Spermidine is a polyamine molecule that performs various cellular functions, such as DNA and RNA stabilization, autophagy modulation, and eIF5A formation, and is generated from putrescine by aminopropyltransferase spermidine synthase (SpdS). During synthesis, the aminopropyl moiety is donated from decarboxylated S-adenosylmethionine to form putrescine, with 5′-deoxy-5′-methylthioadenosine being produced as a byproduct. Spermidine synthase (SpdS; EC 2.5.1.16) is a major type of aminopropyltransferase that converts putrescine into spermidine. In addition, SpdS contains a structural feature known as the gate-keeping loop, which is located in the vicinity of the entrance to the active site.

Here, we determined the crystal structure of an apo-form of SpdS from Kluyveromyces lactis (KlSpdS) at 1.9 Å resolution. KlSpdS exists as a dimer in the asymmetric unit, and each monomer in the dimeric KlSpdS is positioned with two-fold symmetry. Each KlSpdS monomer consists of three domains: an N-terminal domain (residues 4–66), a central catalytic core domain (residues 67–250), and a C-terminal domain (residues 251–292). Meanwhile, the catalytic core domain contains seven β-strands that form a Rossmann-like fold from β7 to β13 and seven α-helices. The electrostatic surface representation of KlSpdS revealed a large cavity in the catalytic core domain between the N- and C-terminal domains; the cavity was highly negatively charged, suggesting that positively charged dcSAM bind to putrescine in this active site pocket. While the gate-keeping loop of H. sapiens SpdS (HsSpdS) sterically hindered the entrance of the active site, that of KlSpdS had an open conformation. In KlSpdS, the α6 helix kinked outward by approximately 41.0° compared to HsSpdS and by approximately 34.6° compared to A. thaliana SpdS (AtSpdS). The catalytic residues Asp98, Asp167, and Asp 170 of KlSpdS were highly conserved in other SpdS structures. Although Asp98 and Asp167 had conformations similar to the other structures, conformation of Asp170 was distinct, possibly due to changes caused by ligand binding. Here, we found that the first structure of fungal KlSpdS, which was determined at 1.9 Å resolution, exhibited highly similar to that of HsSpdS, suggesting that KlSpdS is phylogenetically closer to HsSpdS than SpdS from E. coli and could therefore utilize a sequential mechanism rather than a ping-pong mechanism.

>[2x]MSELTHPTIVDGWFREISDTMWPGQAMTLRVEKILHHEKSKYQDVLVFKSTDYGNVLVLDNAIQVTERDEFSYQEMIAHLALNSHPNPKKVLVIGGGDGGVLREIVKHDSVQEAWLCDIDEAVIRVSKEYLPEMAKSYSHPKVKTHIGDGFQFLRDYQNTFDVIITDSSDPEGPAASLFQQSYFELLNGALTEKGVISTQAESMWIHLPIIKELKKACKEVFPTVGYAYTTIPTYPTGQIGFMVCSKDANVDVTKPLRSISEEEEEAKYRYYNKKVHEASFVLPTWVAKELDL> MSGFNFGAASAGGFSFGNPKSTTTTAPTGFSFGAATAAPSGGFSFGTATPTPASTTGQTSGLFSFSNPAPSLAPTSGFSFGAQVTSTPAPSSGGLAFGANTSKLNSGVGNQPAGGTTQTSQPMGGFSFGAATTQTQPSATSVGGFSFAGGVGSTSTNVFAQPAASTGITLQSAVSTAAAPTATTSQPTSTFSFGTQPQAAPALNFGLLSSSSVLSTASTPAAAQPVAPTTGLSLNFGKPADTSAAVTSTGSTTTNTPSLSSLLGTSGPSLFSSVATSTVPSVVSTVASGLSLTSTATSTGFGMKTLASSAVPTGTLATSTASLGVKAPLAGTIVQANAVGSAAATGISTATAMTYAQLENLINKWSLELEDQEKHFLQQATQVNAWDRTLMQN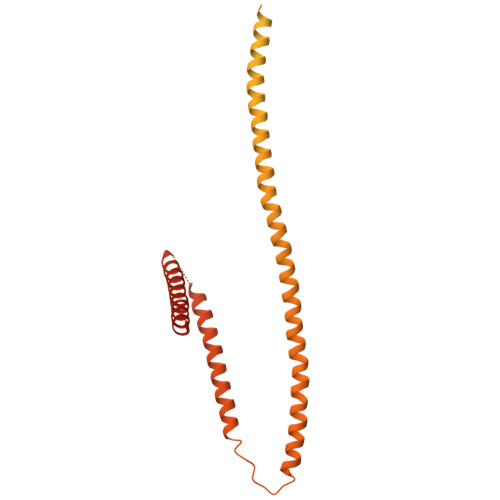GERITTLHREMEKVKLDQKRLDQELDFILSQQKELEDLLTPLEESVKEQSGTIYLQHADEEREKTYKLAENIDAQLKRMAQDLKEVIEHLNTSAGPGDASNPLQQICKILNAHMDSLQWIDQNSALLQRKVEQVTKECESRRKEQERGFSIAFD> GPGSNSKNPVPVKKEAKLSEAELHDKIKNLEEEKAELFEKLDKVEEEHKKVEEEHKKDHEKLEKKSEDVERHYLRQLDQEYKEQQERQKNLEELE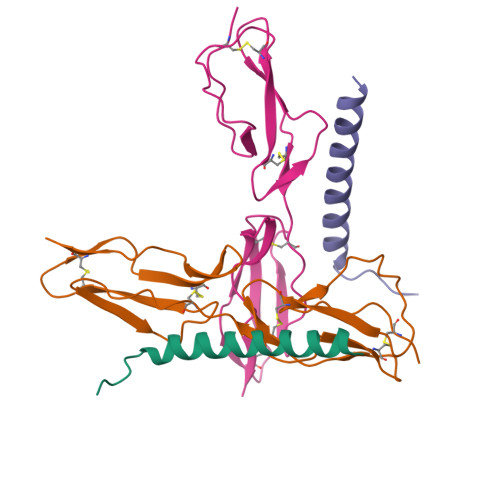RQSQREVEKR;> GPGSNCGPPPTLSFAAPMDITLTETRFKTGTTLKYTCLPGYVRSHSTQTLTCNSDGEWVYNTFCIYKRCRHPGELRNGQVEIKTDLSFGSQIEFSCSEGFFLIGSTTSRCEVQDRGVGWSHPLPQCEI> SMPVKTGSPTFVRELRSRTFDSSDEVILKPTGNQLTVEFLEENSFSVPILVLKKDGLGMTLPSPSFTVRDVEHYVGSDKEIDVIDVTRQADCKMKLGDFVKYYYSGKREKVLNVISLEFSDTRLSNLVETPKIVRKLSWVENLWPEECVFERPNVQKYCLMSVRDSYTDFHIDFGGTSVWYHVLKGEKIFYLIRPTNANLTLFECWSSSSNQNEMFFGDQVDKCYKCSVKQGQTLFIPTGWIHAVLTPVDCLAFGGNFLHSLNIEMQLKAYEIEKRLSTADLFRFPNFETICWYVGKHILDIFRGLRENRRHPASYLVHGGKALNLAFRAWTRKEALP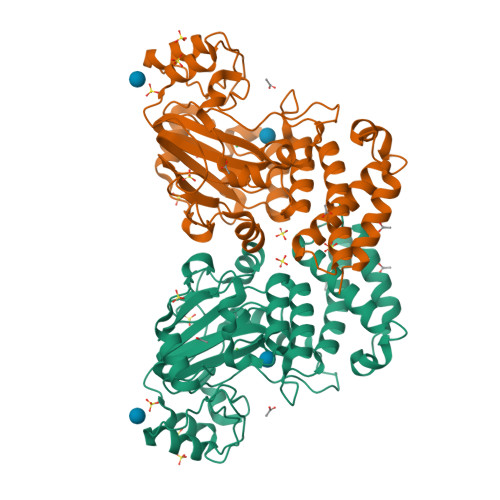DHEDEIPETVRTVQLIKDLAREIRLVEDIFQQN> MQDPDGIDINTKIFNSVAEVFQKAQGSYAGHRKHIAVLKKIQSKAVEQGYEDAFNFWFDKLVTKILPLKKNEIIGDRIVKLVAAFIASLERELILAKKQNYKLTNDEEGIFSRFVDQFIRHVLRGVESPDKNVRFRVLQLLAVIMDNIGEIDESLFNLLILSLNKRIYDREPTVRIQAVFCLTKFQDEEQTEHLTELSDNEENFEATRTLVASIQNDPSAEVRRAAMLNLINDNNTRPYILERARDVNIVNRRLVYSRILKSMGRKCFDDIEPHIFDQLIEWGLEDRELSVRNACKRLIAHDWLNALDGDLIELLEKLDVSRSSVCVKAIEALFQSRPDILSKIKFPESIWKDFTVEIAFLFRAIYLYCLDNNITEMLEENFPEASKLSEHLNHYILLRYHHNDISNDSQSHFDYNTLEFIIEQLSIAAERYDYSDEVGRRSMLTVVRNMLALTTLSEPLIKIGIRVMKSLSINEKDFVTMAIEIINDIRDDDIEKQEQEEKIKSKKINRRNETSVDEEDENGTHNDEVNEDEEDDNISSFHSAVENLVQGNGNVSESDIINNLPPEKEASSATIVLCLTRSSYMLELVNTPLTENILIASLMDTLITPA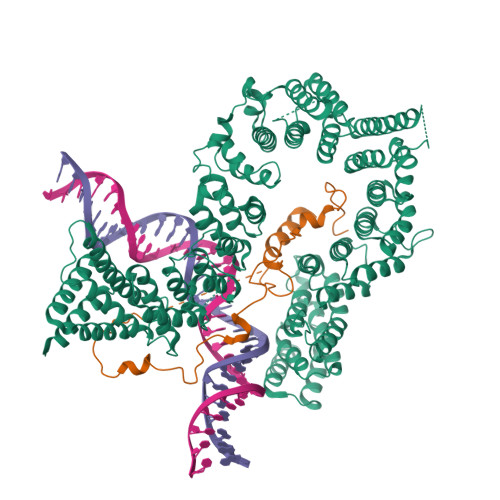VRNTAPNIRELGVKNLGLCCLLDVKLAIDNMYILGMCVSKGNASLKYIALQVIVDIFSVHGNTVVDGEGKVDSISLHKIFYKVLKNNGLPECQVIAAEGLCKLFLADVFTDDDLFETLVLSYFSPINSSNEALVQAFAFCIPVYCFSHPAHQQRMSRTAADILLRLCVLWDDLQSSVIPEVDREAMLKPNIIFQQLLFWTDPRNLVNQTGSTKKDTVQLTFLIDVLKIYAQIEKKEIKKMIITNINAIFLSSEQDYSTLKELLEYSDDIAENDNLDNVSKNALDKLRNNLNSLIEEINERSETQTKDENNTANDQYSSILGNSFNKSSNDTIEHAADITDGNNTELTKTTVNISAVDNTTEQSNSRKRTRSEAEQIDTSKNLENMSIQDTSTVAKNVSFVLPDEKSDAMSIDEEDKDSESFSEVC;> MTTQLRYENNDDDERVEYNLFTNRSTMMANFEEWIKMATDNKINSRNSWNFALIDYFYDLDVLKDGENNINFQKASATLDGCIKIYSSRVDSVTTETGKLLSGLAQRKTNGASNGDDSNGGNGEGLGGDSDEANIEIDPLTGMPISNDPDVNNTRRRVYNRVLETTLVEFETIKMKELDQELIIDPLFKKALVDFDEGGAKSLLLNTLNIDNTARVIFDASIKDTQNVGQGKLQRKEEELIERDSLVDDENEPSQSLISTRNDSTVNDSVISAPSMEDEILSLGMDFIKFDQIAVCEISGSIEQLRNVVEDINQAKDFIENVNNRFDNFLTEEELQAAVPDNAEDDSDGFDMGMQQELCYPDENHDNTSHDEQDDDNVNSTTGSIFEKDLMAYFDENLNRNWRGREHWKVRNFKKANLVNKESDLLEETRTTIGDTTDKNTTDDKSMDTKKKHKQKKVLEIDFFKTDDSFEDKVFASKGRTKIDMPIKNRKNDTHYLLPDDFHFSTDRITRLFIKPAQKMSLFSHRKHTRGDVSSGLFEKSTVSANHSNNDIPTIADEHFWADNYERKEQEEKEKEQSKEVGDVVGGALDNPFEDDMDGVDFNQAFEGTDDNEEASVKLDLQDDEDHKFPIRENKVTYSRVSKKVDVRRLKKNVWRSINNLIQEHDSRKNREQSSNDSETHTEDESTKELKFSDIIQGISKMYSDDTLKDISTSFCFICLLHLANEHGLQITHTENYNDLIVNYEDLATTQAASLVGGGHHRPHHGGHHHHHHGGRIFYPYDVPDYAGYPYDVPDYAGSYPYDVPNYAAGH(8S,11R,13S,14S,17S)-11-[4-(dimethylamino)phenyl]-17-(3,3-dimethylbut-1-yn-1-yl)-17-hydroxy-13-methyl-1,2,6,7,8,11,12,13,14,15,16,17-dodecahydro-3H-cyclopenta[a]phenanthren-3-one 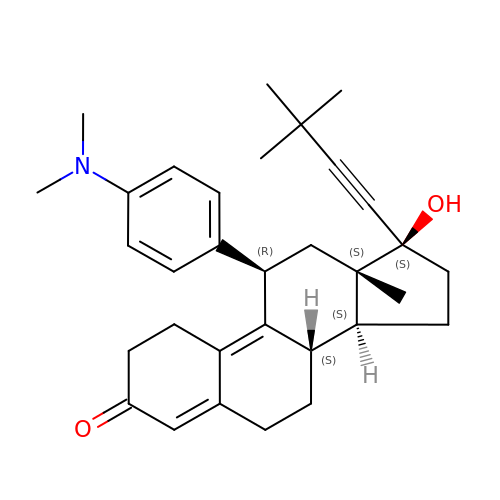(non-preferred name) | C32 H41 N O2 | MKYOYWSMPLRHDW-SSKMXYOESA-N[(2R,5R)-5-(6-aminopurin-9-yl)-4-fluoro-2,5-dihydrofuran-2-yl]oxymethyl-[hydroxy(phosphonooxy)phosphoryl]oxy-phosphinic 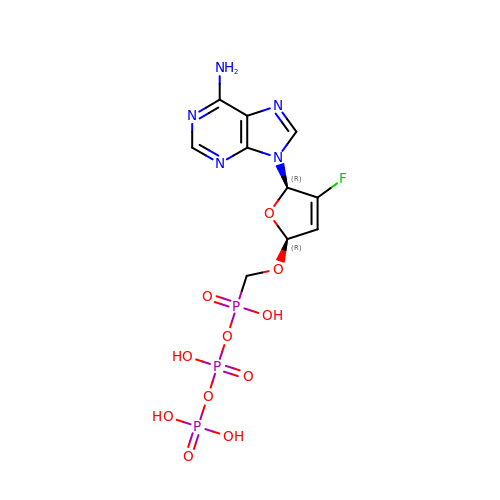acid | C10 H13 F N5 O11 P3 | VWRYHMYAWKXIKG-QUBYGPBYSA-N>MLKQVEIFTDGSCLGNPGPGGYGAILRYRGREKTFSAGYTRTTNNRMALMAAIVALEALKEHCEVILSTDSQYVRQGITQWIHNWKARGWKTADKKPVKNVDLWQRLDAALGQHQIKWEWVKGHAGHPE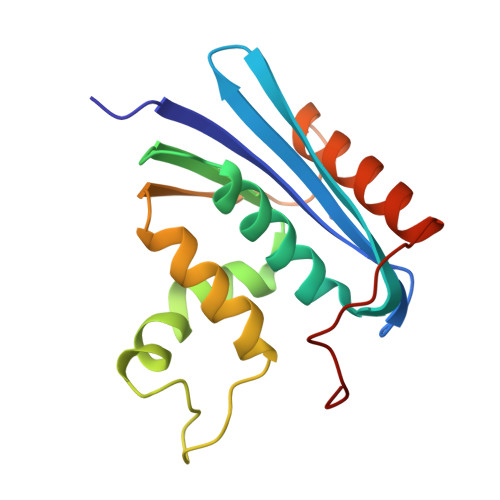NERCNELARAAAMNPTLEDTGYQVEV[4x]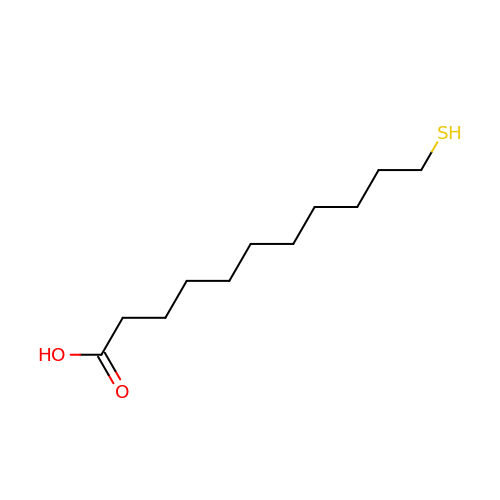11-MERCAPTOUNDECANOIC ACID | C11 H22 O2 S | GWOLZNVIRIHJHB-UHFFFAOYSA-N> MKTTPLVHVASVEKGRSYEDFQKVYN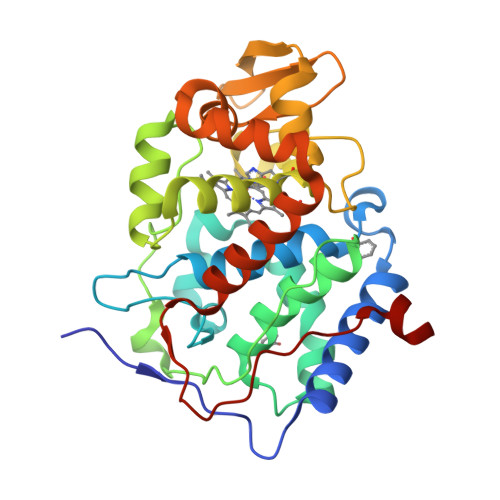AIALKLREDDEYDNAIGYGPVLVRLAWHTSGTWDKHDNTGGSYGGTYRFKKEFNDPSNAGLQNGFKFLEPIHKEFPWISSGDLFSLGGVTAVQEMQGPKIPWRCGRVDTPEDTTPDNGRLPDADKDADYVRTFFQRLNMNDREVVALMGAHALGKTHLKRSGYEGPWGAANNVFTNEFYLNLLNEDWKLEKNDANNEQWDSKSGYMMLPTDYSLIQDPKYLSIVKEYANDQDKFFKDFSKAFEKLLENGITFPKDAPSPFIFKTLEEQGL Mitomycin C (MMC) repair factor A (mrfA) and factor B (mrfB), encode a conserved helicase and exonuclease that repair DNA damage in the soil-dwelling bacterium Bacillus subtilis. MrfB is a member of the DnaQ superfamily of exonucleases with the DEDD motif, which includes the proofreading domains of many DNA polymerases, including Escherichia coli Pol I (polA) and the Pol III ϵ subunit (dnaQ). Using exonuclease assays we show that MrfB is a Mg2+-dependent 3′–5′ DNA exonuclease. The MrfAB pathway responds specifically to MMC insults and works independently of the UvrABC NER process.

The MrfB exonuclease core was purified and initial sparse matrix screens were set with the addition of MgCl2 and dTMP, which would represent the nucleotide product of the exonuclease reaction. The structure was solved by molecular replacement with the AlphaFold model for residues 33–279 as a search model. Two molecules of MrfB were present in the asymmetric unit. The dimeric status in the crystal likely arises from crystal packing as the exonuclease core eluted as a monomer on gel filtration. Density was observed for residues 34–111, 119–202 and 213–279. There was no density observed for dTMP, and only one Mg2+ (site A) was observed at the active site, coordinated by residues Asp107, Glu109 and Asp262. Furthermore, a predicted α-helix from residues 171–183 was in a random coil, which resulted in Asp172 being displaced away from the active site and unable to coordinate a Mg2+ ion in the B site. Because the mechanism for DnaQ exonucleases coordinates two metal ions, we expect that this structure represents an inactive state, and the AlphaFold model likely represents an active state. In the AlphaFold model, Phe171 is poised to base stack with the DNA, and in our structure is instead flipped into a hydrophobic pocket. Instead, we propose this conformation protects hydrophobic residues of MrfB from solvent when it is not engaged with DNA, and it becomes activated upon DNA binding.

>[2x]DDIPFLEEWEAFGMKPFIFEDEYCLIREVEYPLSHRHGLYSFSELEEVITLWNQSGLSHTLSAKGYNKNNLFFFDTETTGLGGGAGNTIFLLGHARVYEDRVTVKQHLLPKPGNEVALYQSFLSEVDITSLVTYNGKAFDWPQVKTRHTLIRDRLPKLPEFGHFDLLHGARRLWKHKMDRVSLGTVEKEELGIRRLEDTPGYLAPMLYFHFIKAQEPDLLKGVLHHNEMDVLSLISLYIHMSKKILS> GSHMNGSKGISPEQEELIHRLVYFQNEYEHPSEEDVKRIINQPMDGEDQCDVRFRHITEITILTVQLIVEFAKRLPGFDKLLREDQIALLKACSSEVMMFRMARRYDVQTDSILFVNNQPYSRDSYNLAGMGETIEDLLHFCRTMYSMRVDNAEYALLTA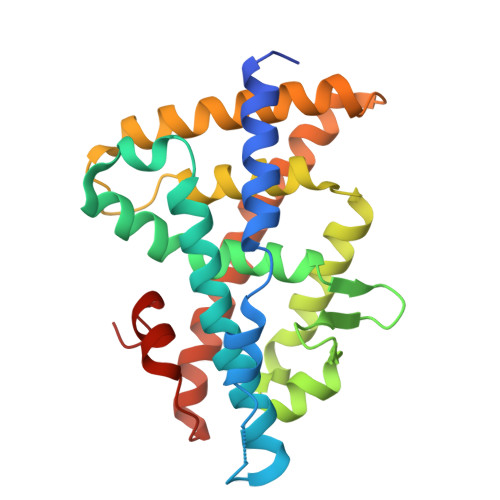IVIFSERPALIEGWKVEKIQEIYLEALRAYVDNRRKPKPGTIFAKLLSVLTELRTLGNQNSEMCFSLKLKNKKLPPFLAEIWDVDLKT ECF transporters consist of two identical or highly similar cytoplasmic ATPases, EcfA and EcfA′, and two transmembrane subunits, EcfT and the S-component124. The membrane-embedded S-component serves as both the substrate-binding and the substrate-translocation domain. The other three subunits (EcfA, EcfA′ and EcfT) together form the ECF module that energizes substrate transport by the S-component456. Here we report crystal structures of the group II ECF transporter for folate from Lactobacillus delbrueckii (L. delbrueckii) in the apo-state and in complex with the slowly hydrolysable ATP analogue AMP–PNP.

In addition, we present a structure of solitary FolT from the same organism in the folate-bound state. We determined the crystal structure of folate-bound FolT1 at 3.0 Å resolution. Well-defined non-protein electron density inside the α-helical core was assigned to the folate molecule. The occluded folate-binding site is lined by all six membrane α-helices and is located close to the extracellular side of the membrane (orientation as in Fig. 1a), where it is shielded from the exterior by the L1 loop connecting helices 1 and 2, and the L3 loop between helices 3 and 4. The substrate-binding pocket has a volume of about 1,400 Å3, which leaves a vast amount of space for extensions on the folate molecule such as a polyglutamate tail. The pterin moiety of the folate molecule forms a network of strong interactions with residues from helices 3 and 4, and the connecting loop L3, while the aminobenzoate and glutamate moieties interact with residues from helices 5 and 6, and loop L1. A detailed description of the interactions is provided in the supplement, but it is important to note that loop L1 and loop L3 provide many of the interactions with the folate molecule. In FolT1, L1 and L3 cover the folate-binding pocket and provide multiple interactions with the substrate, whereas they have moved away in the substrate-free state, creating a wide opening. The conformations of loops L1 and L3 in folate-bound FolT1 are incompatible with binding to the ECF module, because they would clash with TMH3 of the membrane domain of EcfT at the position of the conserved P71. Thus, high-affinity binding of folate to FolT and interaction of EcfT with FolT are mutually exclusive.

>HHHHHHHHMKSESKVSSKLELRELVLLAMVIAIKVVLGQFKVGDATLQVGLGFIGSVMLGYLFGPWWGFAGGALSDLVSSAIFGNLGGFFIGFTLTAALESMIYGFFLYKKPIQIWRVIASVICVTVICYIGLNTLWVSMLGGTNFMVALSSRILKEMITPWIHMVVVWFILEGLSRVKLSRKF[2x]ADENOSINE-5'-MONOPHOSPHATE-PROPYL ESTER | 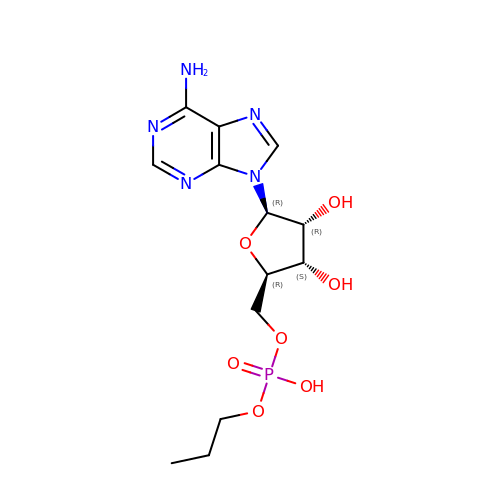C13 H20 N5 O7 P | XAMXMSZRQHPMRX-QYVSTXNMSA-N>[2x]MLLFPFESRSRSIPTGGWQMKRAWWKESVVYQIYPRSFQDSNGDGIGDIPGIVSRLDYL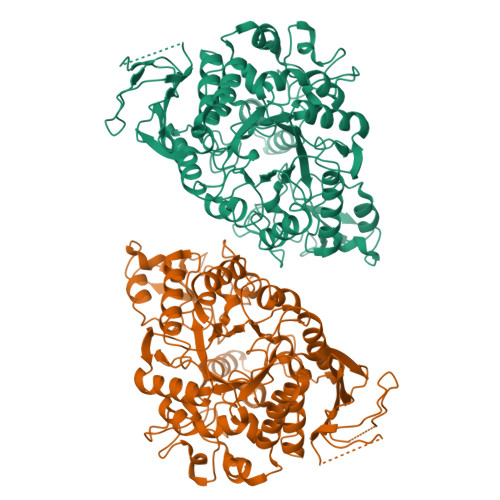QELGVDVVWLCPVYDSPNDDNGYDIRDYRRIMDEFGTLEDWERLLEDLHARGMKLIMDLVVNHSSDEHAWFSESRKSRDGEHRDYYIWRDGKGGAEPNNWSSFFSGSAWKYDGETDQYYLHLFSSKQPDLNWENGKVRREVYNMMAWWLDKGIDGFRMDVINLISKVPGLPDAPGEGRYRSGADYFMNGPRVHEYLQEMNREVLSRYDIMTVGETPGVTPEQAALYVGEDRGELNMVFQFEHMDIDSGPGGKWDVQPWRLTDFKRVMGKWQRELQDRGWNSLYLNNHDQPRMVSRFGDDKNFRKQSAKMLGTLLHTLQGTPYIYQGEELGMTNVRFGSIEDYRDIETLNMYKEATGAGRPAEAVMASVYSKGRDNARTPMQWDGSAHGGFTTGTPWIASNPNYTEINAEDARRDPDSIFHYYRRLIALRKQHDVIVYGRYEALLEEDERIYAYTRMLDGERLLVVLNFFGEEADCSLPEKIRFESAEPLIGNYGNGADRDWRSLKLRPYEALVLRLQG>[2x]GAEIPKEMLRAQTNXILLNVLKQGDNYVYGIIKQVKEASNGEMELNEATLYTIFKRLEKDGIISSYWGDESQGGRRKYYRLTEIGHENMRLAFES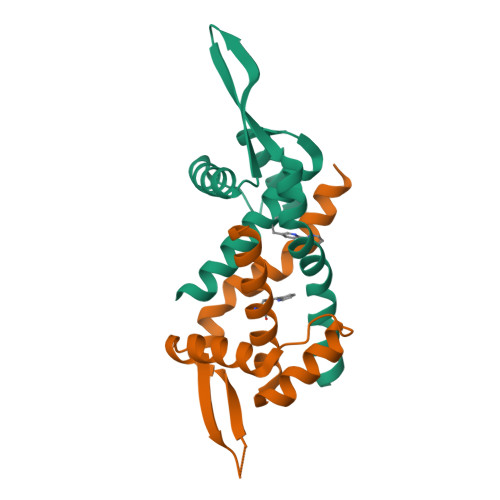WSRVDKIIENLEANKKSEAIKSRGGSGGWSHPQFEK>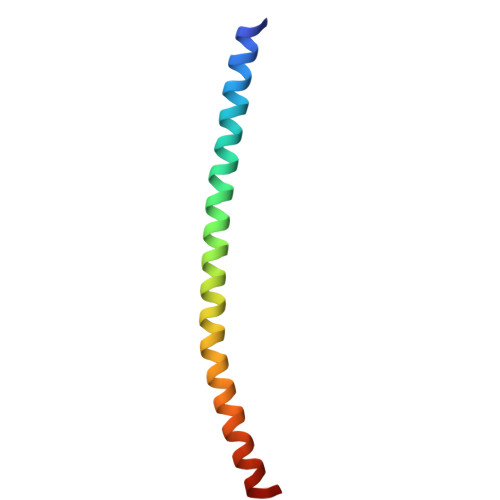 SELLQRCESLEKKTATFENIVCVLNREVERVAMTAEACSRQHRLDQDKIEALSSKVQQLERSIGLE In a subset of nontypeable strains, the major nonpilus adhesin is a protein called Hia. Hia contains two homologous binding domains, called HiaBD1 and HiaBD2, that interact with the same host cell receptor. In particular, the Hia passenger domain consists of repeats of structurally similar domains, including five structurally identical Trp-ring domains strung together by two IsNeck domains and two KG domains.

To investigate this issue and to clarify the structural determinants of Hia-mediated binding, we determined the structures of two Hia passenger domain fragments: one with adhesive activity (Hia51–166, corresponding to HiaBD2, which shares a 45% sequence identity with HiaBD1), and the other with no adhesive function (Hia307–422, which shares an 18% sequence identity with HiaBD1). The structure of HiaBD2 was determined to a resolution of 2.0 Å, using molecular replacement and HiaBD1 as search model. HiaBD2 contains two well-defined structural domains, namely, IN1 and W1. IN1 is a globular knob-like domain with a simple α/β sandwich fold. In the trimer, αIN14 from each HiaBD2 subunit forms a three-helix bundle parallel with the axis of the trimer from which the three knob-like shapes protrude laterally. The W1 domain of HiaBD2 is an all-β domain consisting of five long β-strands (βW11–βW15). In the trimer, these strands are highly intertwined, forming a five-stranded β-sheet on each face of the trimer and serving as a surface against which the αIN12 and αIN13 helices of IN1 rest. The structures of HiaBD2 and HiaBD1 are very similar, aligning with a root mean square deviation (RMSD) in Cα positions of 1.1 Å between IN1 of HiaBD2 and IN2 of HiaBD1, and 1.5 Å between W1 of HiaBD2 and W5 of HiaBD1 (see superposition of the two structures in Fig. 3a). However, due to the lack of structural information on HiaBD2, it was not clear which residues account for this difference in adhesive activity. The examination of the binding groove described above reveals only one notable difference among functionally important residues between HiaBD1 and HiaBD2 in this region, namely, D618 in HiaBD1 corresponds to a glutamine residue in HiaBD2, resulting in a change in charge and a longer side chain. We propose that the distal binding domain (HiaBD2/HsfBD2) initiates the initial interaction with the host cell surface.

>[3x]NNTPVTNKLKAYGDANFNFTNNSIADAEKQVQEAYKGLLNLNEKNASDKLLVEDNTAATVGNLRKLGWVLSSKNGTRNEKSQQVKHADEVLFEGKGGVQVTSTSENGKHTITFALA> MLQKRIPQIICTLLLLGSFSQIKAQDRVPFDQGKKYTLAKVSVVGKISFNEQTVVTFSGLQKGQEITVPGEEITSAIKKLGKLGLFDEIAFYINKVENDSIYLDLNIVELPKLNEVKITGVKKSKVEGLIKDNNLTKNKIVNENLITTTKNYIENKYKKDGFYNTKVVITTTPDTTAGNQVNMLVRVDKGDKVKISSIDFTGNKQLSDSKLRAAMKDTKQKNVLRVFKASKFIPEKYKTDLEKVIASYKEKGYRDARIIYDSVIYNKKKNMLAIKIDVEEGNKYYFGNIKFLGNTVYSDQQLNRYLGIKKGETYNGVLLE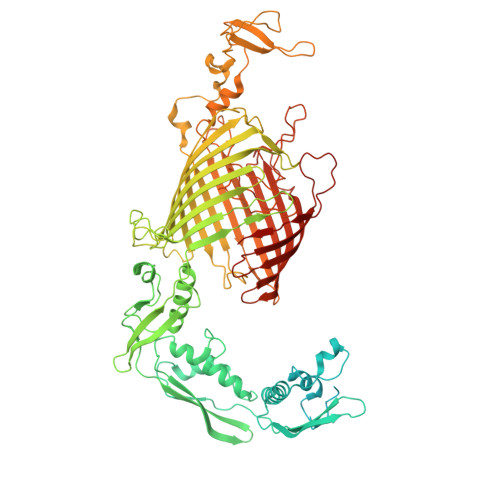KRIADNTKPDGEDITNLYQNNGYLFSKINAVEVKTVNDTIDFEIRITEGPIAYFNKIYVTGNDKTNDHVIYRELRTKPGNKYSKEELVRTIREIGQLGFFDPESIKPEFRNVDPAAGTVDIEYQLVEKGSSQVELQGGYGGGGFIGTLGLSFNNFSARKLFDKDAYKPLPMGDGQKVALRLQGSTYFQTYSLSFSEPWFGGKKPVQFSSSISYSKQFNYNYSSRDVNRNQSFNIFTVQVGLAKRLTVPDDYFVLSQSVSYQHYDLNNYYTGLFTFGNGASRNLAYTIGLSRSNKGVNPIFPTYGSEFSISAKVTPPYSLFNNINYGDLQNQKEYKTQYTGTTTTTGIDGQAINPGDYTKTETVNGQSGTVSVGSDYKSADTDVGKVDQKKYNWLEYYKVKFKADWYTKIYGKLVLRTLTEFGFLGAYDQSRGVVPFERFYLGGDGMANYSMDGRETIQLRGYPNNSLTPIIEDRNSSRYGQQIGATIYNKFSMELRYPITLKSSASIYALTFLEAGSSYPTFKDYNPFDLNRSAGAGLRVFMPAFGLLGIDFGYGFDALPGSTTNKANGWETHFIIGQQF> MFRASCTLLGHGQYKTRLKKRMVGFIPKVIPRKIRNNMVALRSEANTGHMEGYIKTEAERLDATGRKLQ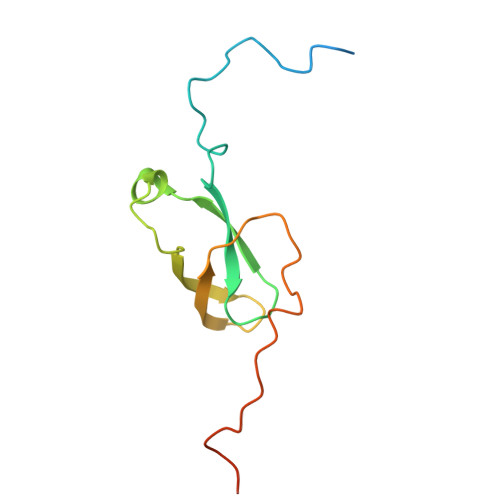KTMWDPVLQRYTLMKETKVRGPFLTKSNIARKVDFPVGALHGTKLGGKK>[2x]MKDDFAKLEEQFDAKLGIFALDTGTNRTVAYRPDERFAFASTIKALTVGVLLQQKSIEDLNQRITYTRDDLVNYNPITEKHVDTGMTLKELADASLRYSDNAAQNLILKQIGG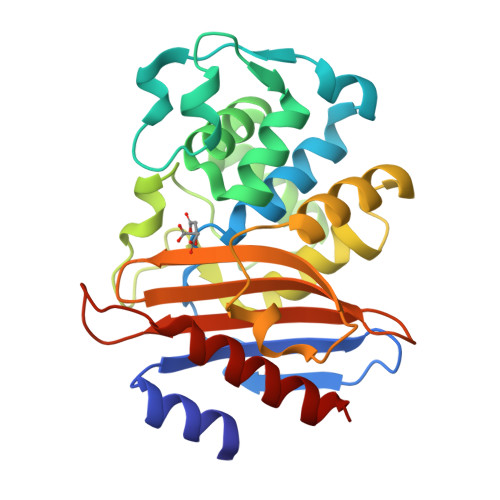PESLKKELRKIGDEVTNPERFEPELNEVNPGETQDTSTARALVTSLRAFALEDKLPSEKRELLIDFMKRNTTGDALIRAGVPDGFEVADKTGAASYGTRNDIAIIFPPKGDPVVLAVLSSRDKKDAKYDDKLIAEATKVVMKALN> MNEHYTESDIKRNHKTEKNKTEKEKFKDSINNLVKTEFTNETLDKIQQTQDLLKKIPKDVLEIYSELGGEIYFTDIDLVEHKELQDLSEEEKNSMNSRGEKVPFASRFVFEKKRETPKLIINIKDYAINSEQSKEVYYEIGKGISLDIISKDKSLDPEFLNLIKSLSDDSDSSDLLFSQKFKEKLELNNKSIDINFIKENLTEFQHAFSLAFSYYFAPDHRTVLELYAPDMFEYMNKLEKGGFEKISESLKKEGVEKDRIDVLKGEKALKASGLVPEHADAFKKIARELNTYILFRPVNKLATNLIKSGVATKGLNVHGKSSDWGPVAGY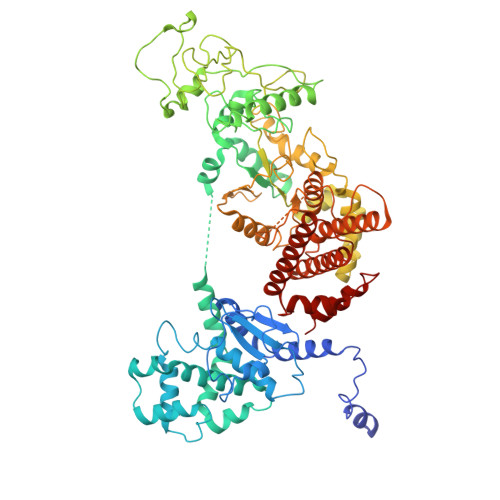IPFDQDLSKKHGQQLAVEKGNLENKKSITEHEGEIGKIPLKLDHLRIEELKENGIILKGKKEIDNGKKYYLLESNNQVYEFRISDENNEVQYKTKEGKITVLGEKFNWRNIEVMAKNVEGVLKPLTADYDLFALAPSLTEIKKQIPQKEWDKVVNTPNSLEKQKGVTNLLIKYGIERKPDSTKGTLSNWQKQMLDRLNEAVKYTGYTGGDVVNHGTEQDNEEFPEKDNEIFIINPEGEFILTKNWEMTGRFIEKNITGKDYLYYFNRSYNKIAPGNKAYIEWTDPITKAKINTIPTSAEFIKNLSSIRRSSNVGVYKDSGDKDEFAKKESVKKIAGYLSDYYNSANHIFSQEKKRKISIFRGIQAYNEIENVLKSKQIAPEYKNYFQYLKERITNQVQLLLTHQKSNIEFKLLYKQLNFTENETDNFEVFQKIIDEK> SSLDDKPQFPGASAEFIDKLEFIQPNVISGIPIYRVMDRQGQIINPSEDPHLPKEKVLKLYKSMTLLNTMDRILYESQRQGRISFYMTNYGEEGTHVGSAAALDNTDLVFGQYREAGVLMYRDYPLELFMAQCYGNISDLGKGRQMPVHYGCKERHFVTISSPLATQIPQAVGAAYAAKRANANRVVICYFGEGAASEGDAHAGFNFAATLECPIIFFCRNNGYAISTPTSEQYRGDGIAARGPGYGIMSIRVDGNDVFAVYNATKEARRRAVAENQPFLIEAMTYRIGHASTSADSSAFRSVDEVNYWDKQDHPISRLRHYLLSQGWWDEEQEKAWRKQSRRKVMEAFEQAERKPKPNPNLLFSDVYQEMPAQLRKQQESLARHLQTYGEHYPLDHFDK;> VAHFTFQPDPEPREYGQTQKMNLFQSVTSALDNSLAKDPTAVIFGEDVAFGGVFRCTVGLRDKYGKDRVFNTPLCEQGIVGFGIGIAVTGATAIAEIQFADYIFPAFDQIVNEAAKYRYRSGDLFNCGSLTIRSPWGCVGHGALYHSQSPEAFF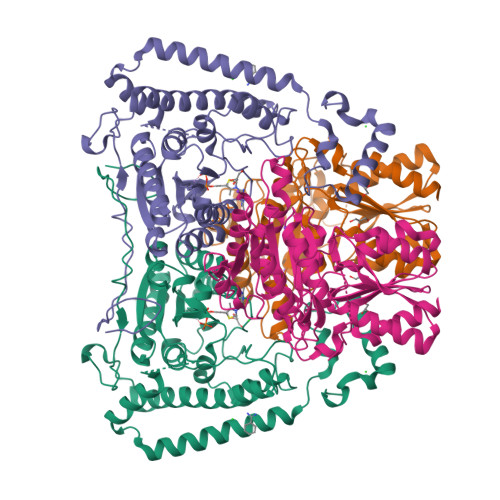AHCPGIKVVIPRSPFQAKGLLLSCIEDKNPCIFFEPKILYRAAAEEVPIEPYNIPLSQAEVIQEGSDVTLVAWGTQVHVIREVASMAKEKLGVSCEVIDLRTIIPWDVDTICKSVIKTGRLLISHEAPLTGGFASEISSTVQEECFLNLEAPISRVCGYDTPFPHIFEPFYIPDKWKCYDALRKMINY>[5x]QELGNANFENFIGATEGFSEIAYQFTSAILTLGYAVMLAGLLYFILTIKNVDKKFQMSNILSAVVMVSAFLLLYAQAQNWTSSFTFNEEVGRYFLDPSGDLFNNGYRYLNWLIDVPMLLFQILFVVS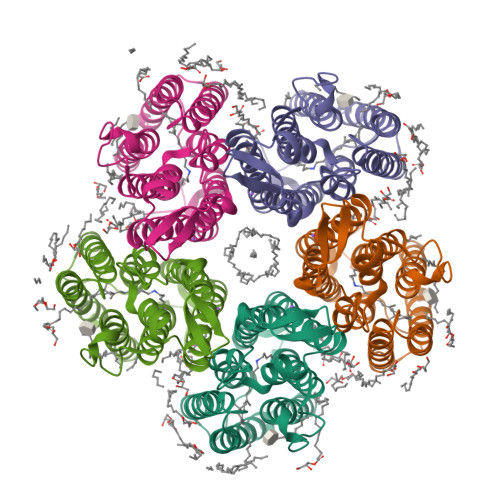LTTSKFSSVRNQFWFSGAMMIITGYIGQFYEVSNLTAFLVWGAISSAFFFHILWVMKKVINEGKEGISPAGQKILSNIWILFLISWTLYPGAYLMPYLTGVDGFLYSEDGVMARQLVYTIADVSSKVIYGVLLGNLAITLSKNKEL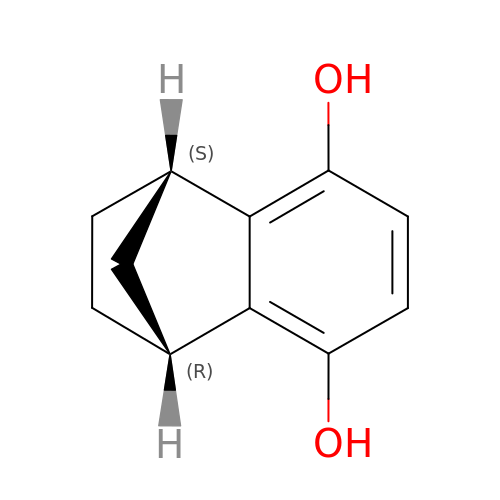(1R,4S)-1,2,3,4-tetrahydro-1,4-methanonaphthalene-5,8-diol | C11 H12 O2 | JYHNNCBQCSLFQM-KNVOCYPGSA-N>[2x]MAHHHHHHGHHHQLSEDSELIEQVIEQPDSLIISPPSDSSSSSYNHIQPFVYLESTATTQTNHNVLLILNQKITID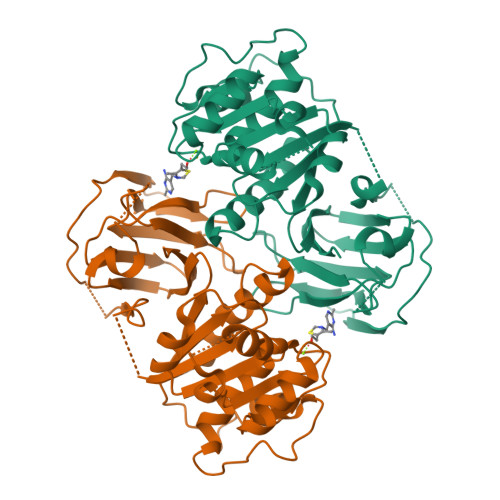LISLWKKCEIIVCADGGANSLYEYFNDNNHHHHHENLQRSDYIPDYIVGDFDSISPDVKTYYESHGSKIIRQSSQYYNDFTKSIHCIQLHYQLNHTKENWFESIDEVDGLAKLWNGLNNSSDVVVDIDITIYVLNAIGGRFDQTVQSINQLYIMNEDYPKVTVFFITTNDIIFLLKKGVNYISYKNRLMFHKDNGSSPTPTCGLLPLSNKTPIILNSYGLKYDMRNWKTEMLGQVSSSNRISGETGFIVECSDDIVMNIEIDV> A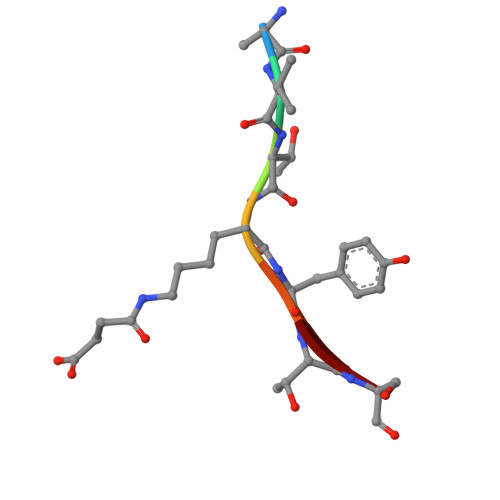VTXYTS>MRLCDRDIEAWLDEGRLSINPRPPVERINGATVDVRLGNKFRTFRGHTAAFIDLSGPKDEVSAALDRVMSDEIVLDEGEAFYLHPGELALAVTLESVTLPADLVGWLDGRSSLARLGLMVHVTAHRIDPGWSGCIVLAFYNSGKLPLALRPGMLIGALSFEPLSGPAVRPYNRREDAKYRNQ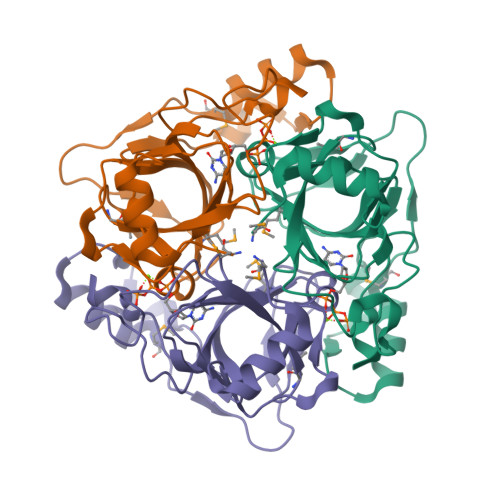QGAVASRIDKD[6x]> NRCCDR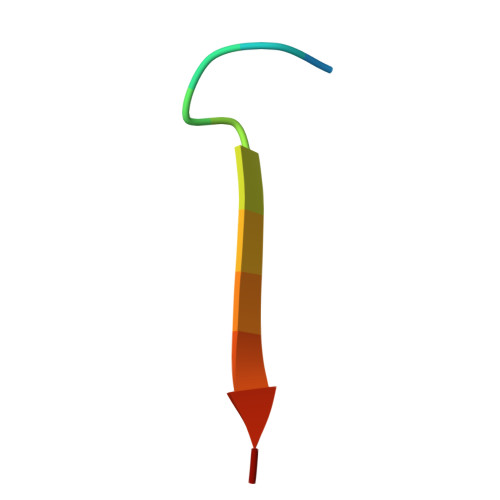YEEYDLE> MTWLPLNPIPLKDRVSMIFLQYGQIDVIDGAFVLIDKTGIRTHIPVGSVACIMLEPGTRVSHAAVRLAAQVGTLLVWVGEAGVRVYASGQPGGARSDKLLYQAKLALDEDLRLKVVRKMFELRFGEPAPARRSVEQLRGIEGSRVRATYALLAKQYG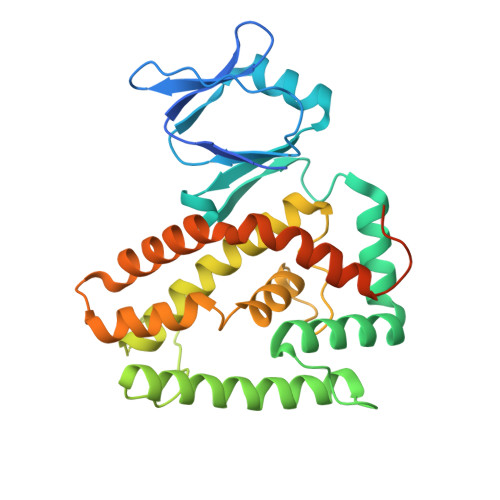VTWNGRRYDPKDWEKGDTINQCISAATSCLYGVTEAAILAAGYAPAIGFVHTGKPLSFVYDIADIIKFDTVVPKAFEIARRNPGEPDREVRLACRDIFRSSKTLAKLIPLIEDVLAAGEIQPPAPPEDAQPVAIPLPVSLGDAGHRSS> SNAPPGTVDKKMVEKCWKLMDKVVRLCQNPKLALKNSPPYILDLLPDTYQHLRTILSRYEGKMETLGENEYFRVFMENLMKKTKQTISLFKEGKERMYEENSQPRRNLTKLSLIFSHMLAELKGIFPSGLFQGDTFRITKADAAEFWRKAFGEKTIVPWKSFRQALHEVHPISSGLEAMALKSTIDLTCNDYISVFEFDIFTRLFQPWSSLLRNWNSLAVTHPGYMAFLTYDEVKA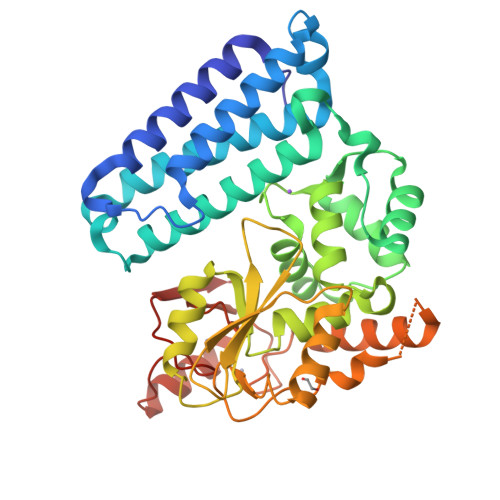RLQKFIHKPGSYIFRLSCTRLGQWAIGYVTADGNILQTIPHNKPLFQALIDGFREGFYLFPDGRNQNPDLTGLCEPTPQDHIKVTQEQYELECEMGSTFQLCKICAENDKDVKIEPCGHLMCTSCLTSWQESEGQGCPFCRCEIKGTEPIVVDPFD>MSSGVPVLLFKEGTSRNSGRDALKNNILAARTLAEMLRSSLGPKGLDKMLIDSFGDVTITNDGATIVKEMEIQHPAAKLLVEAAKAQDSEVGDGTTSAVVLAGLFLEKAESLVDQNIHPTIIIEGFKKAFNKSLELLPQLATKVDVSDLNSATARDALKKIVYTTMSSKFMAEGEELNKIMDIVIDAVTTVAEPLPDGGYNVSLDLIKIDKKKGGTIEDSQLIRGIVLDKEVVHAGMPRRVEKAKIAVLDASLEVEKPEISAKISITSPDQIKAFLDEEAKYLKDMVDKLASIGANVVICQKGIDDIAQHFLAKRGILAVRRVKRSDIEKLEKALGARIISSIKDATPEDLGYAELVEERKVGNDKMVFIEGAKNPKAVNILLRGSNDMALDEAERSINDALYSLRNILMEPYIVPGGGAIELELSARLREYARSVGGKEQLAIEAYADALEEIPMILAETAGLEPISALMDLRARHAKGLTNCGVDVINGKIIDDIYSINVVEPIRVTRQVLKSATEAATSIMKIDDLIAASQLKSSGKGAGAGAGGEGAEG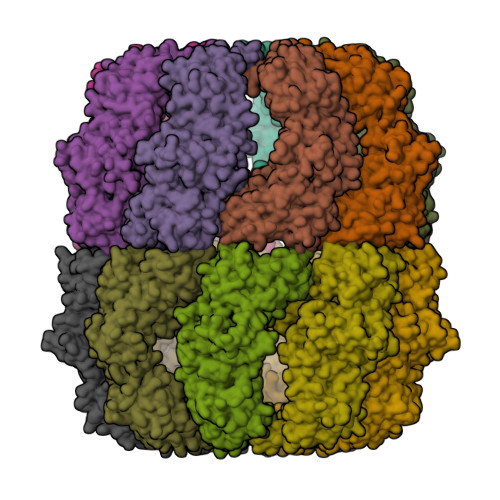GGAPSMEGLS[16x]>[2x]MSENNKNSLESSLRQLKCHFTWNLME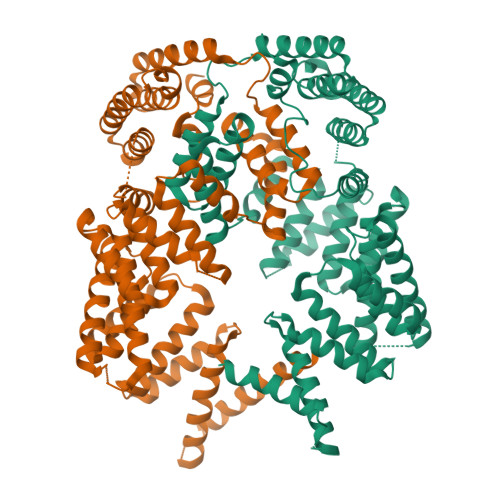GENSLDDFEDKVFYRTEFQNREFKATMCNLLAYLKHLKGQNEAALECLRKAEELIQQEHADQAEIRSLVTWGNYAWVYYHMGRLSDVQIYVDKVKHVCEKFSSPYRIESPELDCEEGWTRLKCGGNQNERAKVCFEKALEKKPKNPEFTSGLAIASYRLDNWPPSQNAIDPLRQAIRLNPDNQYLKVLLALKLHKMREEGEEEGEGEKLVEEALEKAPGVTDVLRSAAKFYRRKDEPDKAIELLKKALEYIPNNAYLHCQIGCCYRAKVFQVMNLRENGMYGKRKLLELIGHAVAHLKKADEANDNLFRVCSILASLHALADQYEEAEYYFQKEFSKELTPVAKQLLHLRYGNFQLYQMKCEDKAIHHFIEGVKINQKSREKEKMKDKLQKIAKMRLSKNGADSEALHVLAFLQELNEKMQQADEDSERGLESGSLIPSASSWNGE> MRALLPYLALYKRHKWMLSLGIVLAIVTLLASIGLLTLSGWFLSASAVAGVAGLYSFNYMLPAAGVRGAAITRTAGRYFERLVSHDATFRVLQHLRIYTFSKLLPLSPAGLARYRQGELLNRVVADVDTLDHLYLRVISPLVGAFVVIMVVTIGLSFLDFTLAFTLGGIMLLTLFLMPPLFYRAGKSTGQNLTHLRGQYRQQLTAWLQGQAELTIFGASDRYRTQLENTEIQWLEAQRRQSELTALSQAIMLLIGALAVILMLWMASGGVGGNAQPGALIALFVFCALAAFEALAPVTGAFQHLGQVIASAVRISDLTDQKPEVTFPDTQTRVADRVSLT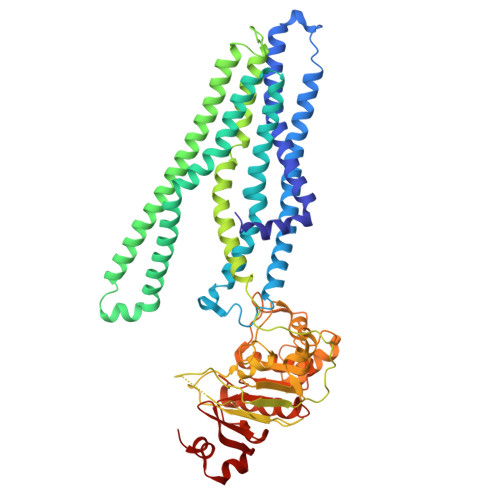LRDVQFTYPEQSQQALKGISLQVNAGEHIAILGRTGCGKSTLLQQLTRAWDPQQGEILLNDSPIASLNEAALRQTISVVPQRVHLFSATLRDNLLLASPGSSDEALSEILRRVGLEKLLEDAGLNSWLGEGGRQLSGGELRRLAIARALLHDAPLVLLDEPTEGLDATTESQILELLAEMMREKTVLMVTHRLRGLSRFQQIIVMDNGQIIEQGTHAELLARQGRYYQFKQGL>[2x]MAATTVNGGTVHFKGEVVNAACAVDAGSVDQTVQLGQVRTASLAQEGATSSAVGFNIQLNDCDTNVASKAAVAFLGTAIDAGHTNVLALQSSAAGSATNVGVQILDRTGAALTLDGATFSSETTLNNGTNTIPFQARYFATGAATPGAANADATFKVQYQ;> MGVALGATRVIYPAGQKQEQLAVTNNDENSTYLIQSWVENADGVKDGRFIVTPPLFAMKGKKENTLRILDATNNQLPQDRESLFWMNVKAIPSMDKSKLTENTLQLAIISRIKLYYRPAKLALPPDQAAEKLRFRRSANSLTLINPTPYYLTVTELNAGTRVLENALVPPMGESTVKLPSDAGSNITYRTINDYGALTPKMTGVME;> DLYFNPRFLADDPQAVADLSRFENGQELPPGTYRVDIYLNNGYMATRDVTFNTGDSEQGIVPCLTRAQLASMGLNTASVAGMNLLADDACVPLTTMVQDATAHLDVGQQRLNLTIPQAFMSNRARGYIPPELWDPGINAGLLNYNFSGNSVQNRIGGNSHYAYLNLQSGLNIGAWRLRDNTTWSYNSSDRSSGSKNKWQHINTWLERDIIPLRSRLTLGDGYTQGDIFDGINFRGAQLASDDNMLPDSQRGFAPVIHGIARGTAQVTIKQNGYDIYNSTVPPGPFTINDIYAAGNSGDLQVTIKEADGSTQIFTVPYSSVPLLQREGHTRYSITAGEYRSGNAQQEKPRFFQSTLLHGLPAGWTIYGGTQLADRYRAFNFGIGKNMGALGALSVDMTQANSTLPDDSQHDGQSVRFLYNKSLNESGTNIQLVGYRYSTSGYFNFADTTYSRMNGYNIETQDGVIQVKPKFTDYYNLAYNKRGKLQLTVTQQLGRTSTLYLSGSHQTYWGTSNVDEQFQAGLNTAFEDINWTLSYSLTKNAWQKGRDQMLALNVNIPFSHWLRSDSKSQWRHASASYSMSHDLNGRMTNLAGVYGTLLEDNNLSYSVQTGYAGGGDGNSGSTGYATLNYRGGYGNANIGYSHSDDIKQLYYGVSGGVLAHANGVTLGQPLNDTVVLVKAPGAKDAKVENQTGVRTDWRGYAVLPYATEYRENRVALDTNTLADNVDLDNAVANVVPTRGAIVRAEFKARVGIKLLMTLTHNNKPLPFGAMVTSESSQSSGIVADNGQVYLSGMPLAGKVQVKWGEEENAHCVANYQLPPESQQQLLTQLSAECRLVPRGSWSHPQFEK

Uropathogenic Escherichia coli strains use filamentous type 1 pili to adhere to and invade uroepithelial cells. The pilus consists of a flexible tip fibrillum, formed by the adhesin FimH and the subunits FimG and FimF. The pilus rod is a helical assembly of up to 3000 copies of the main subunit FimA, terminated by a single copy of the subunit FimI that anchors the rod to the assembly platform FimD in the outer membrane. The assembly platform FimD in the outer membrane of uropathogenic E. coli is the catalyst of type 1 pilus assembly.

The assembly conditions were further optimized to produce a sample with an average pilus length suitable for cryo-EM, allowing us to determine the overall structure of the FimDHGFAnC complex to 4.1 Å resolution. However, the rod was initially not well-resolved due to its flexible connection between subunit FimAn-1 occupying the pore and FimAn-2 emerging from the pore. Multi-body refinement in RELION-5.033,34 further enhanced the resolutions, yielding 3.6 Å for the pilus rod (body 1) and 3.9 Å for the assembly platform (body 2). By combining the maps of the two bodies, we constructed a composite map that includes both the assembly platform and pilus rod, which sits at an approximately 51° angle on top of the usher. On the periplasmic side of FimD, the FimAn-FimC complex is bound to the CTDs, while the preceding subunit, FimAn-1, occupies the pore of the usher. The NTD is unoccupied and not well-resolved. Multi-body refinement provided insights into the movement of the pilus rod relative to the assembly platform. Although restrained by the rim of the β-barrel and the extracellular loops of FimD, principal component analysis revealed a twisting motion of up to 11°, as well as side-to-side and back-and-forth motions of up to 19° and 18°, respectively. Multi-body analysis indicates that the connection between FimAn-1 and FimAn-2 serves as the main pivot point for pilus rod motion relative to the usher.> MKKINGWIVVALLAVTTVGAAAAIQYTNNADSPGQF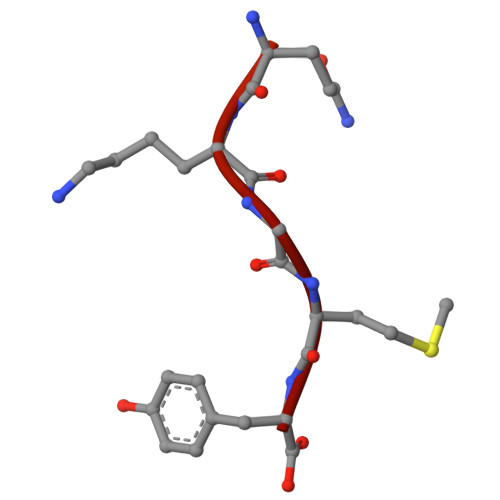QVAQKGMY Leucyl-tRNA synthetase (LRS), a class I AaRS, is particularly large and complex. Structurally, LRS contains an aminoacylation domain, a tRNA binding domain, and an editing domain, known as connective peptide 1 (CP1). HcLRS functions as the intracellular leucine sensor to modulate the activity of the mTOR complex 1 (mTORC1) by directly binding with RagD GTPase, the mediator of the AAs-dependent mTORC1 pathway. After screening truncations with different lengths, we found that deletion of the last 106 residues (N1071-1176C), designated as hcLRS_d106, gives improved crystals that diffract up to 2.5 Å resolution.

We were able to obtain a co-crystal structure of hcLRS bound with a tavaborole derivative, a previous reported anti-cryptosporidium benzoxaborole, AN6426 (37). The structure was refined to 3.0 Å resolution. The IC50 of AN6426 to hcLRS in vitro is 7.7 μM. In the structure, AN6426-AMP is well accommodated in the editing pocket with the AN6426 moiety mainly binding to residues from the editing active site, such as Thr293, Thr298 and Asp399. The side chain of Lys 464 from the I4ae insertion is within the Van der Waals interaction distance with the ether group at the meta-C of AN6426. Structurally, this I4ae insertion makes the size of editing pocket from hcLRS much smaller than those from bacteria LRSs. One could imagine that if we added a bigger group to the meta-C of AN6426, this group will clash with the I4ae insertion of hcLRS. So it is theoretically feasible to design benzoxaborole-based derivatives with larger groups that will target bacteria LRSs but are too big for hcLRS. Taken together, our results showed that it is feasible to design benzoxaborole-based derivatives targeting specifically LRS from bacterial microbes but not hcLRS.

>MGHHHHHHHHHHSSGHIEGRHMMAERKGTAKVDFLKKIEKEIQQKWDTERVFEVNASNLEKQTSKGKYFVTFPYPYMNGRLHLGHTFSLSKCEFAVGYQRLKGKCCLFPFGLHCTGMPIKACADKLKREIELYGCPPDFPDEEEEEEETSVKTEDIIIKDKAKGKKSKAAAKAGSSKYQWGIMKSLGLSDEEIVKFSEAEHWLDYFPPLAIQDLKRMGLKVDWRRSFITTDVNPYYDSFVRWQFLTLRERNKIKFGKRYTIYSPKDGQPCMDHDRQTGEGVGPQEYTLLKLKVLEPYPSKLSGLKGKNIFLVAATLRPETMFGQTNCWVRPDMKYIGFETVNGDIFICTQKAARNMSYQGFTKDNGVVPVVKELMGEEILGASLSAPLTSYKVIYVLPMLTIKEDKGTGVVTSVPSDSPDDIAALRDLKKKQALRAKYGIRDDMVLPFEPVPVIEIPGFGNLSAVTICDELKIQSQNDREKLAEAKEKIYLKGFYEGIMLVDGFKGQKVQDVKKTIQKKMIDAGDALIYMEPEKQVMSRSSDECVVALCDQWYLDYGEENWKKQTSQCLKNLETFCEETRRNFEATLGWLQEHACSRTYGLGTHLPWDEQWLIESLSDSTIYMAFYTVAHLLQGGNLHGQAESPLGIRPQQMTKEVWDYVFFKEAPFPKTQIAKEKLDQLKQEFEFWYPVDLRVSGKDLVPNHLSYYLYNHVAMWPEQSDKWPTAVRANGHLLLNSEKMSKSTGNFLTLTQAIDKFSADGMRLALADAGDTVEDANFVEAMADAGILRLYTWVEWVKEMVANWDSLRSGPASTFNDRVFASELNAGIIKTDQNYEKMMFKEALKTGFFEFQAAKDKYRELAVEGMHRELVFRFIEVQTLLLAPFCPHLCEHIWTLLGKPDSIMNASWPVAGPVNEVLIHSSQYLMEVTHDLRLRLKNYMMPAKGKKTDKQPLQKPSHCTIYVAKNYPPWQHTTLSVLRKHFEANNGKLPDNKVIASELGSMPELKKYMKKVMPFVAMIKENLEKMGPRILDLQLEFDEKAVLMENIVYLTNSLELEHIEVKFASEAEDKIREDCCPGKPLNVFRIEPGVSVS[2x]> MQTVNEMLRRAATRAPDHCALAVPARGLRLTHAELRARVEAVAARLHADGLRPQQRVAVVAPNSADVVIAI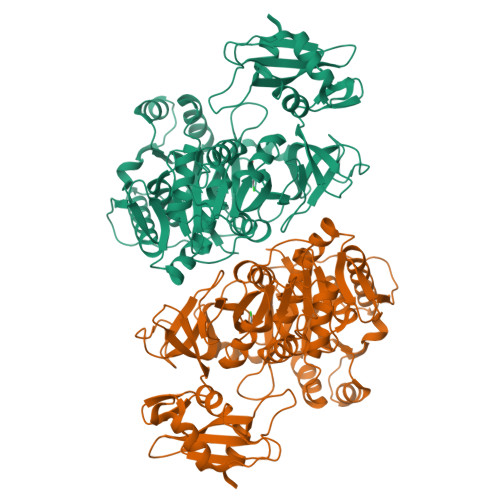LALHRLGAVPALLNPRLKSAELAELIKRGEMTAAVIAVGRQVADAIFQSGSGARIIFLGDLVRDGEPYSYGPPIEDPQREPAQPAFIFYTSGTTGLPKAAIIPQRAAESRVLFMSTQVGLRHGRHNVVLGLMPLYHVVGFFAVLVAALALDGTYVVVEEFRPVDALQLVQQEQVTSLFATPTHLDALAAAAAHAGSSLKLDSLRHVTFAGATMPDAVLETVHQHLPGEKVNIYGTTEAMNSLYMRQPKTGTEMAPGFFSEVRIVRIGGGVDEIVANGEEGELIVAASDSAFVGYLNQPQATAEKLQDGWYRTSDVAVWTPEGTVRILGRVPDMIISGGENIHPSEIERVLGTAPGVTEVVVIGLADQRWGQSVTACVVPRLGETLSADALDTFCRSSELADFKRPKRYFILDQLPKNALNKVLRRQLVQQVSS> SPTINFINFNQTGTCISLGTSKGFKIFNCEPFGKFYSEDSGGYAIVEM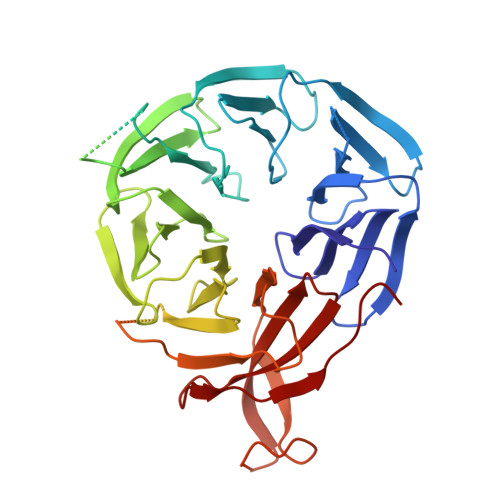LFSTSLLALVGIGDQPALSPRRLRIINTKKHSIICEVTFPTSILSVKMNKSRLVVLLQEQIYIYDINTMRLLHTIETNPNPRGLMAMSPSVANSYLVYPSPPKVINSEIKAHATTNNITLSVGGNTETSFKRDQQDAGHSDISDLDQYSSFTKRDDADPTSSNGGNSSIIKNGDVIVFNLETLQPTMVIEAHKGEIAAMAISFDGTLMATASDKGTIIRVFDIETGDKIYQFRRGTYATRIYSISFSEDSQYLAVTGSSKTVHIFKLGHSMSNNKLDSDDSNMEEAAADDSSLDTTSIDALSDEENPTRLAREPYVDASRKTMGRMIRYSSQKLSRRAARTLGQIFPIKVTSLLESSRHFASLKLPVETNSHVMTISSIGSPIDIDTSEYPELFETGNSASTESYHEPVMKMVPIRVVSSDGYLYNFVMDPERGGDCLILSQYSILM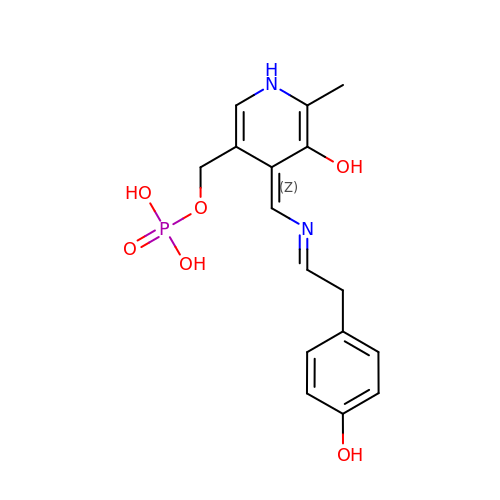[(4Z)-4-[[(Z)-2-(4-hydroxyphenyl)ethylideneamino]methylidene]-6-methyl-5-oxidanyl-1H-pyridin-3-yl]methyl dihydrogen phosphate | C16 H19 N2 O6 P | DXNWHWZTDLTPAE-VHWRWSQTSA-N>[8x]MSKPQPIAAANWKCNGSQQSLSELIDLFNSTSINHDVQCVVASTFVHLAMTKERLSHPKFVIAAQNAIAKS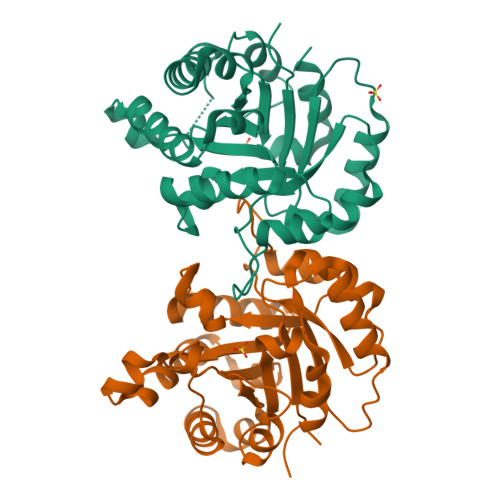GAFTGEVSLPILKDFGVNWIVLGHSERRAYYGETNEIVADKVAAAVASGFMVIACIGETLQERESGRTAVVVLTQIAAIAKKLKKADWAKVVIAYEPVWAIGTGKVLTPQQAQEAHALIRSWVSSKIGADVAGELRILYGGSVNGKNARTLYQQRDVNGFLVGGASLKPEFVDIIKATQ> MGQVLPLVTRQGDRIAIVSGLRTPFARQATAFHGIPAVDLGKMVVGELLARSEIPAEVIEQLVFGQVVQMPEAPNIAREIVLGTGMNVHTDAYSVSRACATSFQAVANVAESLMAGTIRAGIAGGADSSSVLPIGVSKKLARVLVDVNKARTMSQRLKLFSRLRLRDLMPVPPAVAEYSTGLRMGDTAEQMAKTYGITREQQDALAHRSHQRAAQAWSDGKLKEEVMTAFIPPYKQPLVEDNNIRGNSSLADYAKLRPAFDRKHGTVTAANSTPLTDGAAAVILMTESRAKELGLVPLGYLRSYAFTAIDVWQDMLLGPAWSTPLALERAGLTMSDL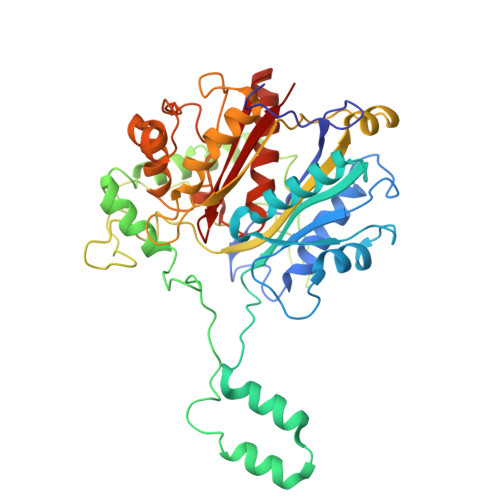TLIDMHEAFAAQTLANIQLLGSERFAREALGRAHATGEVDDSKFNVLGGSIAYGHPFAATGARMITQTLHELRRRGGGFGLVTACAAGGLGAAMVLEAE> GGWIRNIGRYLSYLVDDTFEEYAYDVVDGIAKARTQEELLEGVYKALRLAPKLKKKAESKGCPPPRIPSPEDIEALEEKVEQLSNP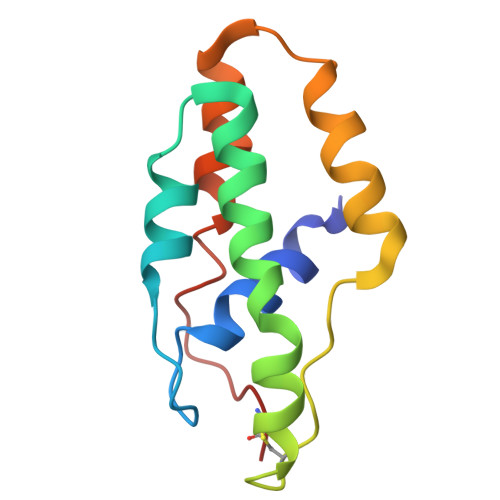KDLRKLAVSLALWAFASWNNCP>[6x]GS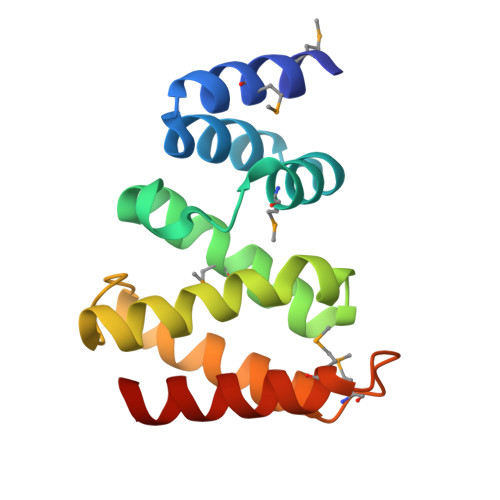HMLWSQAMESVRASDFDLAYADILGSNDELLLVRLMSRTGPVLEQLSDATLTHLMGNLKHFLQQQSFLECVIPWIQQVADLVLSNGPNALGLTGDSKKDLVFALQEAASMDHAQSWMAAKIVELAEQLRSAWL> MCAQPTASTVEGLFKPSSAFADRTDFSLSSILQKSLINRESFNQYLAMRLAPVLRTFYEDNYDTDIKERLNGFTADTDNAFVSQEQNLRNQFRENYLVHLQTDIFDNTGGNQAAWKLRDVNNKIIDDFISRIFAKNFVEYVQDGVGPLTKPTKSLIENTSNFKNIKLQPKFVNKNAKLKINNDAVYAAIQDKLLDQFITNENPNLVSRVVFTNETPVDGFDNYFNTKVIQSPTPSYQFQVFNKYNQQSGGTKGANGFNLLASNLKSYKNDQSKGIDIPNKFSSDSGGKLLLKASDMFDTFDPSFSAAFIQGYLALQKKSKGADSKEVDSLIKDKSIIENFFVDNNT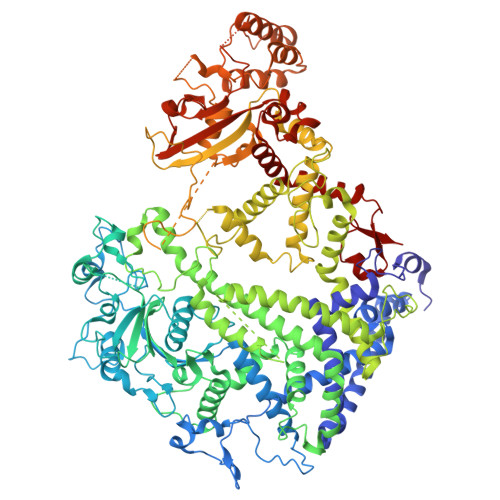QAAAAARAASSSSEGTIQLKTASDGGGTTQSTVHKTDLVKIFGDKDVFAGEYKQQIGNTNANQTGGGGSGGGGGTSTGSSTGSSTETTTGNSSKAVVDLIEVKKDSSSQPDYILSRGKDGIHLMAVDGGSHYLTESGRDVAKQKKFLLFRALQTKYGLVDTDTTYDFKLFDEVKKYFDTNRILFLFEALLDLSSDTNNKDNFLSYPQFKKFADSIKSIEKDLKELVQAHYKQAVFNETAVAENKVTLKLAERNQPFIDNERNNQIEQNGLAAKLPYEQDAKTGHYNDLGNYYKDIIDNVDKKGTSTVKTTSSNTGQTKNFSEEVVSKLKDNKKKVEEAAKKHVEALKVFTIPSPLYSQVILVQTKLSFTPESTSLGLNLALNNYLTSTELQNSIKLSYFQEDEAFKKIIDITNLTFSQQSGGTGGTNGNNNLTADNWKIFKETYLLDLFESQAQKSIFGHVGSSDKNSSTKTGIEGVLDTLYSSLNLEERLDSDDVIDYLSYLYTAHWLLKDNLKNYKQSLQSKLSRTSNAFLVWSVDSEKNKNDSQSTLSSTASSTSNTGLIQLRSVVSLAQNQAAGQGGDNNSDITQTEVKNPNFVFGSSVYDWTNSKTPEVNRAADDTSSFFYTKSSSSSTGAAQSSATVLRSLNQASGMTTKTAKNRYGFRGIVTSSTSGSLPEAVSRRLFKQFVNQTEKGVKVGGQMLITTAKSGKATLVLKQQADDAESTTNNAYKGALFSFGSMDNLKNIINGIQTQTEFDALYNHLTSDLNIDVTGVDKNKTLTEQKTSLTSFVDSNFKQSTQSAQRGDTSARSARSATVQIKKTQEDNQNTNYKDVFSRFDGYIGDNKVEEKNYTSYQFLSDGGKYHATFVKQVNLDDVEKIGTDSLKQEDSSKDKRLNLSLEEFLAAIALEALDPNNQTQAINALISGNKKGLVKVGDFRIFSSISAQWVRRFAAALEHHHHHH> MGSLVREWVGFQQFPAATQEKLIEFFGKLKQKDMNSMTVLVLGKGGVGKSSTVNSLIGEQVVRVSPFQAEGL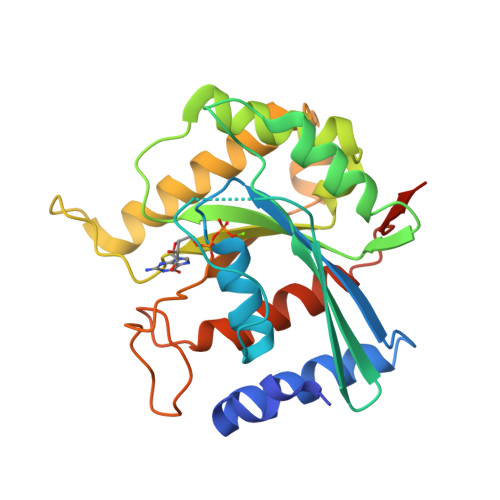RPVMVSRTMGGFTINIIDTPGLVEAGYVNHQALELIKGFLVNRTIDVLLYVDRLDVYRVDELDKQVVIAITQTFGKEIWCKTLLVLTHAQFSPPDELSYETFSSKRSDSLLKTIRAGSKMRKQEFEDSAIAVVYAENSGRCSKNDKDEKALPNGEAWIPNLVKAITDVATNQRKAIHVDAAALEHHHHHH>MRGSHHHHHHGSSHANINAFKEAVTKIDRVEINRRLELAYAYNASIAGAKTNGEYPALKDPYSAEQKQAGVVEYARMLEVKEQIGHVIIPRINQDIPIYAGSAEENLQRGVGHLEGTSLPVGGESTHAVLTAHRGLPTAKLFTNLDKVTVGDRFYIEHIGGKIAYQVDQIKVIAPDQLEDLYVIQGEDHVTLLTCTPYMINSHRLLVRGKRIPYVEKTVQKDSKT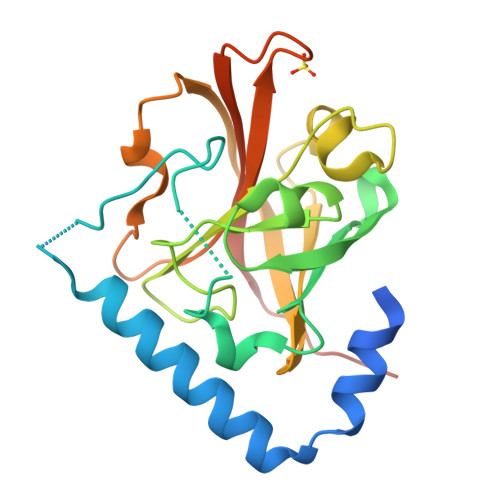FRQQQ[2x]>MQTKKTHLHLISAKASRKYRRTIACLSDTAKKDLERRKQSGAADPAQELSCLKTIKFKLEVPEGSKLPSFDRISQIYNALETIEKGSLSYLLFALILSGFRIFPNSSAAKTFASSSCYKNDQFASQIKEIFGEMVKNFIPSELESILKKGRRKNNKDWTEENIKRVLNSEFGRKNSEGSSALFDSFLSKFSQELFRKFDSWNEVNKKYLEAAELLDSMLASYGPFDSVCKMIGDSDSRNSLPDKSTIAFTNNAEITVDIESSVMPYMAIAALLREYRQSKSKAAPVAYVQSHLTTTNGNGLSWFFKFGLDLIRKAPVSSKQ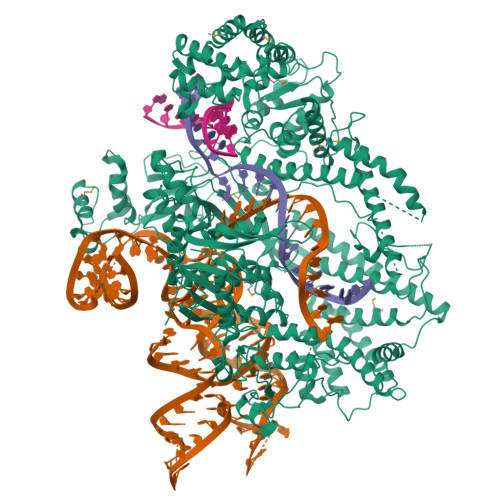STSDGSKSLQELFSVPDDKLDGLKFIKEACEALPEASLLCGEKGELLGYQDFRTSFAGHIDSWVANYVNRLFELIELVNQLPESIKLPSILTQKNHNLVASLGLQEAEVSHSLELFEGLVKNVRQTLKKLAGIDISSSPNEQDIKEFYAFSDVLNRLGSIRNQIENAVQTAKKDKIDLESAIEWKEWKKLKKLPKLNGLGGGVPKQQELLDKALESVKQIRHYQRIDFERVIQWAVNEHCLETVPKFLVDAEKKKINKESSTDFAAKENAVRFLLEGIGAAARGKTDSVSKAAYNWFVVNNFLAKKDLNRYFINCQGCIYKPPYSKRRSLAFALRSDNKDTIEVVWEKFETFYKEISKEIEKFNIFSQEFQTFLHLENLRMKLLLRRIQKPIPAEIAFFSLPQEYYDSLPPNVAFLALNQEITPSEYITQFNLYSSFLNGNLILLRRSRSYLRAKFSWVGNSKLIYAAKEARLWKIPNAYWKSDEWKMILDSNVLVFDKAGNVLPAPTLKKVCEREGDLRLFYPLLRQLPHDWCYRNPFVKSVGREKNVIEVNKEGEPKVASALPGSLFRLIGPAPFKSLLDDCFFNPLDKDLRECMLIVDQEISQKVEAQKVEASLESCTYSIAVPIRYHLEEPKVSNQFENVLAIAQGEAGLAYAVFSLKSIGEAETKPIAVGTIRIPSIRRLIHSVSTYRKKKQRLQNFKQNYDSTAFIMRENVTGDVCAKIVGLMKEFNAFPVLEYDVKNLESGSRQLSAVYKAVNSHFLYFKEPGRDALRKQLWYGGDSWTIDGIEIVTRERKEDGKEGVEKIVPLKVFPGRSVSARFTSKTCSCCGRNVFDWLFTEKKAKTNKKFNVNSKGELTTADGVIQLFEADRSKGPKFYARRKERTPLTKPIAKGSYSLEEIERRVRTNLRRAPKSKQSRDTSQSQYFCVYKDCALHFSGMQADENAAINIGRRFLTALRKNRRSDFPSNVKISDRLLDNLEHHHHHH[2x]>LQTETTDLSLMLEQLTFEFLPLLEEKNLNWQLNLQKNVLATVDTEKIARVF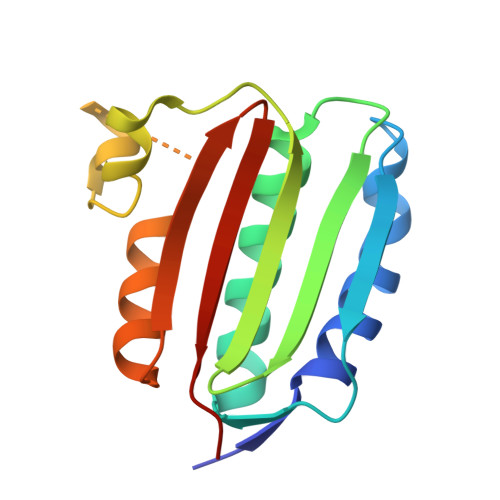DNLIRNAINYSYPDSPLLLELVESDSIHIRLTNRGKTIPEEMIGRLFEPFYRMDSSRATATSGTGLGLPIAKEILLASGGDISAESKDETIIFNVRLPKPANN[2x]>[4x]GVPKLVDHDERRRSITAAAWRLIAARGIEAANMRDIATEAGYTNGALSHYFAGKDEILRTSYEHISEATDRRIAEALGDATGLDALRILCREVMPINEEQLLEARIAASLWPRAMYDE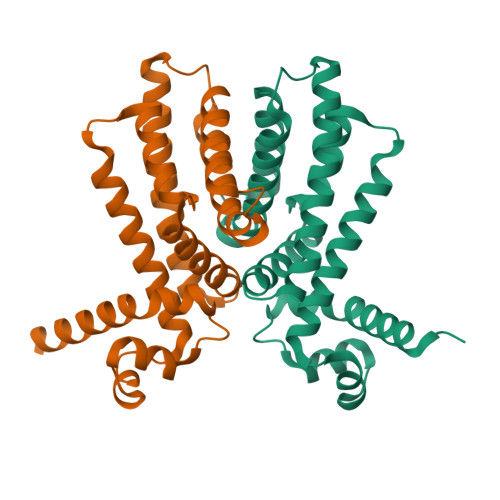QMAATNRRTMDNWREQMAIFLEQAREEGSVGDIDVTIVVEQLLNMMMGMQILGVLTPGETSSERQLEMLEQFVAAL>SMVEDHYEMGEELGSGQFAIVRKCRQKGTGKEYAAKFIKKRRLSSSRRGVSREEIEREVNILREIRHPNIITLHDI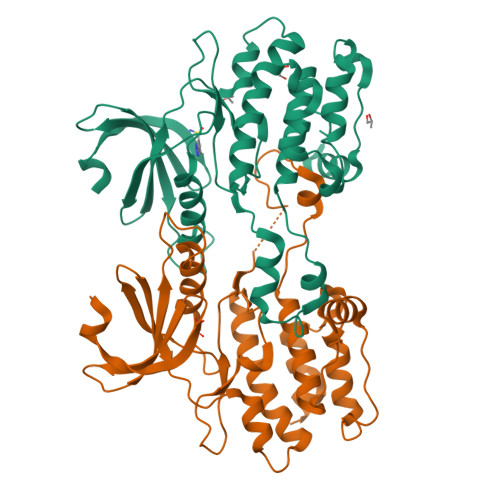FENKTDVVLILELVSGGELFDFLAEKESLTEDEATQFLKQILDGVHYLHSKRIAHFDLKPENIMLLDKNVPNPRIKLIDFGIAHKIEAGNEFKNIFGTPEFVAPEIVNYEPLGLEADMWSIGVITYILLSGASPFLGETKQETLTNISAVNYDFDEEYFSNTSELAKDFIRRLLVKDPKRRMTIAQSLEHSWIKAIRRRNVRGEDSG[2x]PHOSPHONIC ACID | H3 O3 P | 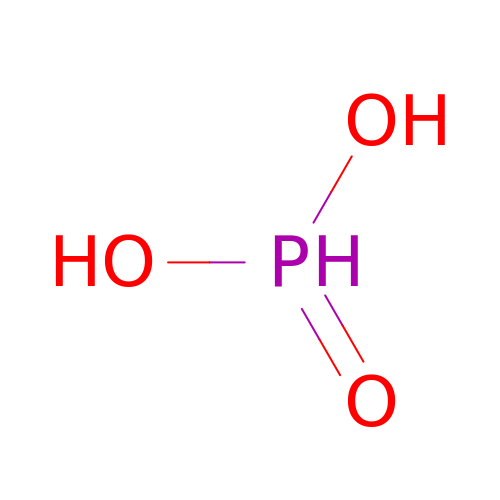ABLZXFCXXLZCGV-UHFFFAOYSA-N Galectin-8 is a tandem-repeat galectin consisting of two distinct carbohydrate recognition domains and is a potential drug target. Like other galectin CRDs, Gal-8N is ~130 amino acid β-sandwich that contains a galectin-defining amino acid motif coordinating conserved binding of galactose via hydrogen bonds to OH 4 and 6, and ring oxygen, and hydrophobic interaction with H 3, 4 and 512. Furthermore, ligands generally bind to the N-terminal domain (Gal-8N) with substantially higher affinity than to the C-terminal domain (Gal-8C). Since the expression of the Gal-8 gene LGALS8 is much more amplified in a variety of tumours compared with Gal-1 and Gal-3, possibly its most important function remains its role in cancer, particularly in angiogenesis and lymphangiogenesis, and inhibiting these processes by a Gal-8 inhibitor seems a plausible therapeutic option.

The alkynyl moiety of the 2-O-propargyl moiety leans directly towards the Arg45 guanidinium group with a distance between the terminal propargyl carbon atom and the terminal Arg45 nitrogen atom of 3.2 Å and 3.4 Å in the two independent copies. However, an even more important answer that could explain the increase in binding enthalpy comes from the structural analysis of 11 in complex with Gal-8N, where a contact between the 2-O-propargyl moiety and a guanidine moiety of Arg45 is observed. This contact is similar to, but not the same as a contact we observed between d-galactal ethylene and the guanidine of Arg45 and may be rationalized by non-canonical cation-π interactions. Alkyne-cation interactions have been reported several times in synthetic chemistry, but to our knowledge no such interactions have been found between a ligand and a protein, which is why we have labelled them “non-canonical cation-π interactions”. These were studied with quantum mechanical calculations which indicate that the LUMO of Arg45 of Gal-8N (depicted in blue) points towards the HOMO electrons of propargyl alkyne (depicted in red) of compound 11, but without evident HOMO-LUMO overlap, meaning that the covalent nature of this interaction is negligible. Yet, the distance between the guanidine C-atom and the terminal C-atom of the alkyne is 3.3 Å, which is in line with a distance threshold for classical cation-π interactions, as these occur within a distance of 6 Å31. The observed interaction is unique and may account for the enthalpy-driven increase in the affinity of 11 for Gal-8N. Surprisingly, the comparison of thermodynamic parameters between 11 and 1 shows an unexpected gain in enthalpic contribution with a further loss in binding entropy compared to 29 (11 vs 1: ΔΔH = –17 kJ mol−1, TΔΔS = +14 kJ mol−1, 11 vs 29: ΔΔH = –4 kJ mol−1, TΔΔS = +6 kJ mol−1), suggesting that contributions other than classical hydrophobic interactions govern the binding of 11.

>[2x]SLNNLQNIIYNPVIPFVGTIPDQLDPGTLIVIRGHVPSDADRFQVDLQNGSSMKPRADVAFHFNPRFKRAGCIVCNTLINEKWGREEITYDTPFKREKSFEIVIMVLKDKFQVAVNGKHTLLYGHRIGPEKIDTLGIYGKVNIHSIGFSFSSD>[6x]GGGHMAIEFDIQESKILKGVYIITPNKFRDLRGEIWTAFTDEYLSKLVPDGIKFKHDKFINSHFNVLRGIHGDVKTYKLVTCVYGEVHQVVVDCRKDSPTYLKWEKFII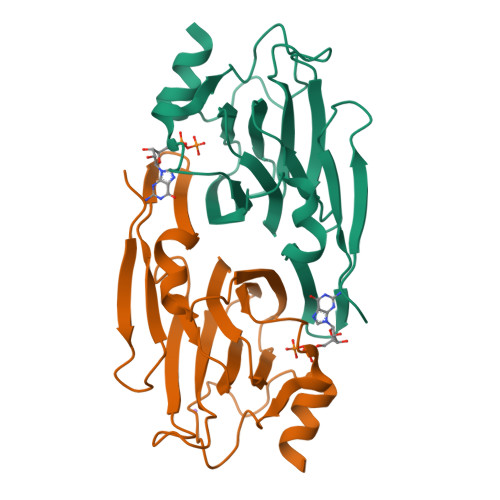SYKNQQLILLPPNMGNSHYVSSAAAVYYYKLAYEGEYMDAPDQFTYAWNDERIGIDWPTNTPILSDRDILATKNKG>SVERIYQKKTQLEHILLRPDTYIGSVELVTQQMWVYDEDVGINYREVTFVPGLYKIFDEILVNAADNKQRDPKMSCIRVTIDPENNLISIWNNGKGIPVVEHKVEKMYVPALIFGQLLTSSNYDDDEKKVTGGRNGYGAKLCNIFSTKFTVETASREYKKMFKQTWMDNMGRAGEMELKPFNGEDYTCITFQPDLSKFKMQSLDKDIVALMVRRAYDIAGSTKDVKVFLNGNKLPVKGFRSYVDMYLKDKLDETGNSLKVIHEQVNHRWEVCLTMSEKGFQQISFVNSIATSKGGRHVDYVADQIVTKLVDVVKKKNKGGVAVKAHQVKNHMWIFVNALIENPTFDSQTKENMTLQPKSFGSTCQLSEK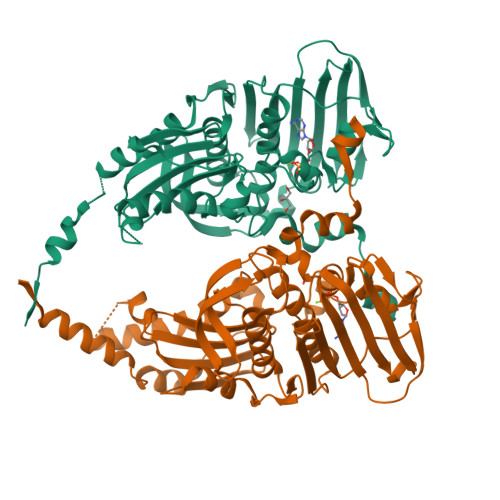FIKAAIGCGIVESILNWVKFKAQVQLNKKCS[4x]>[2x]MSSVTWAPGNYPSTRRSDHVDTYQSASKGEVPVPDPYQWLEESTDEVDKWTTAQADLAQSYLDQNADIQKLAEKFRASRNYAKFSAPTLLDDGHWYWFYNRGLQSQSVLYRSKEPALPDFSKGDDNVGDVFFDPNVLAADGSAGMVLCKFSPDGKFFAYAVSHLGGDYSTIYVRSTSSPLSQASVAQGVDGRLSDEVKWFKFSTIIWTKDSKGFLYQRYPARERHEGTRSDRNAMMCYHKVGTTQEEDIIVYQDNEHPEWIYGADTSEDGKYLYLYQFKDTSKKNLLWVAELDEDGVKSGIHWRKVVNEYAADYNIITNHGSLVYIKTNLNAPQYKVITIDLSKDEPEIRDFIPEEKDAKLAQVNCANEEYFVAIYKRNVKDEIYLYSKAGVQLTRLAPDFVGAASIANRQKQTHFFLTLSGFNTPGTIARYDFTAPETQRFSILRTTKVNELDPDDFESTQVWYESKDGTKIPMFIVRHKSTKFDGTAAAIQYGYGGFATSADPFFSPIILTFLQTYGAIFAVPSIRGGGEFGEEWHKGGRRETKVNTFDDFIAAAQFLVKNKYAAPGKVAINGASNGGLLVMGSIVRAPEGTFGAAVPEGGVADLLKFHKFTGGQAWISEYGNPSIPEEFDYIYPLSPVHNVRTDKVMPATLITVNIGDGRVVPMHSFKFIATLQHNVPQNPHPLLIKIDKSWLGAGMGKPTDKNVKDAADKWGFIARALGLELKTVEMFDTNATRLPIWGIGCNPWTAEHVDQTLASGNDIC;>MFDTNATRLPIWGIGCNPWTAEHVDQTLASGNDIC[2x]

GmPOPB is the macrocyclase responsible for macrocyclization of amatoxins, eight amino-acid ribosomal peptides with the core sequence IWGIGC(N/D)P. Amatoxins are cyclic peptides further modified by a characteristic sulfoxide cross-link between tryptophan and a cysteine, and hydroxylation (the extent of which vary). GmPOPB is an unusual enzyme catalyzing, depending on substrate length, proteolysis, or macrocyclization using the same catalytic machinery. The protein contains two domains as observed in other POP enzymes. The domain containing the putative catalytic residues (Ser577, Asp661, His698) comprises residues 1–81 and 450–728, and the other domain is a seven bladed β-propeller, comprising residues 82–449.

In order to obtain co-complexes, we mutated each residue of the presumed catalytic triad (mutants S577A, D661A, and H698A) to ensure inactive protein. Crystals were obtained for the 35mer complex for S577A and H698A; with the 25mer substrate S577A and D661A. In both 25mer complexes the N-terminal residues of the substrate (IWGIGCN) are disordered; in the S577A–35mer complex the N-terminal two residues (MF) are missing, while in the H698A complex only the first N-terminal residue is absent. There are also no major differences between the H698A–35mer and S577A–35mer complexes, and between the S577A–25mer and D661A–25mer complexes. In the crystal structure of H698A–35mer complex, the hydroxyl of Ser577 is in hydrogen bonding distance from P10, in a position suited for nucleophilic attack but the structure is less ordered, notably the loop containing the mutation H698A. The histidine loop is disordered on the H698A mutant structure and the H698N mutant is insoluble, hinting at a stabilizing role for His698. His698 is 12 Å away (much further than in any other POP) from Ser577 but is essential for catalysis rather than binding. We cannot, however, exclude the possibility that His698 may be required for positioning toward a productive conformation of the enzyme–substrate complex rather than act as a base per se. In the 35mer complex structures, residues 2–9 adopt a helical arrangement that ends up exposed to solvent at the N-terminus and makes few contacts with the protein. To confirm the importance of the putative catalytic triad for GmPOPB, the mutants S577A, D661A, and H698A were evaluated for activity, and were inactive with both 25mer and 35mer substrates, using 5 μM GmPOPB and monitoring the reaction progress after 24 h.> AVTYYRLEEVAKRNTAEETWMVIHGRVYDIT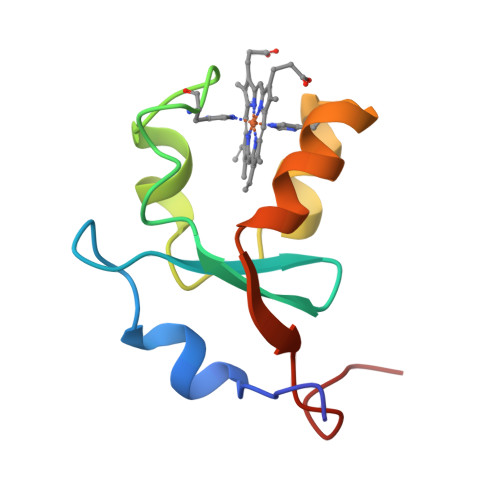RFLSEHPGGEEVLLEQAGADATESFEDVGHSPDAREMLKQYYIGDVHPNDLKP>EPKLDMNKQKISPAEVAKHNKPDDCWVVINGYVYDLTRFLPNHPGGQDVIKFNAGKDVTAIFEPLHAPNVIDKYIAPEKKLGPLQGSMPPELVCPPYAPGETKEDIARKEQLKSLLPPLDNIINLYDFEYLASQTLTKQAWAYYSSGANDEVTHRENHNAYHRIFFKPKILVDVRKVDISTDMLGSHVDVPFYVSATGLCKLGNPLEGEKDVARGCGQGVTKVPQMISTAASCSPEEIIEAAPSDKQIQWYQLYVNSDRKITDDLVKNVEKLGVKALFVTVDAPSLGQREKDMKLKFSNTKAGPKAMKKTNVEESQGASRALSKFIDPSLTWKDIEELKKKTKLPIVIKGVQRTEDVIKAAEIGVSGVVLSNHGGRQLDFSRAPIEVLAETMPIL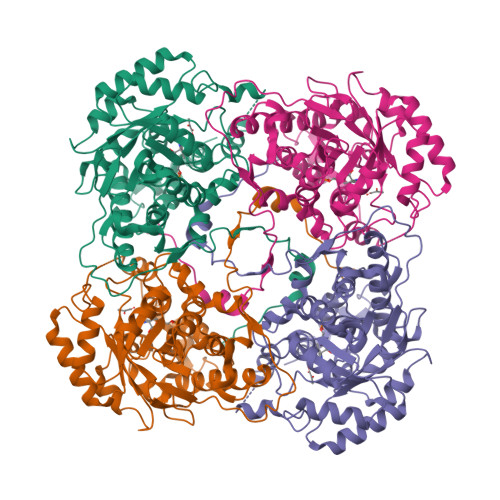EQRNLKDKLEVFVDGGVRRGTDVLKALCLGAKGVGLGRPFLYANSCYGRNGVEKAIEILRDEIEMSMRLLGVTSIAELKPDLLDLSTLKARTVGVPNDVLYNEVYEGPTLTEFEDA[2x]> MGFKSWITEKLNPGQRIIRDMEPVSHRTNRKPFTTGQAYSKIEILNRTANMVIDSAAECSYTVGDKYNIVTYANGVKTKTLDTLLNVRPNPFMDISTFRRLVVTDLLFEGCAYIYWDGTSLYHVPAALMQVEADANKFIKKFIFNNQINYRVDEIIFIKDNSYVCGTNSQISGQSRVATVIDSLEKRSKMLNFKEKFLDNGTVIGLILETDEILNKKLRERKQEELQLDYNPSTGQSSVLILDGGMKAKPYSQISSFKDLDFKEDIEGFNKSICLAFGVPQVLLDGGNNANIRPNIELFYYMTIIPMLNKLTSSLTFFFGYKITPNTKEVAALTPDKEAEAKHLTSLVNNGIITGNEAR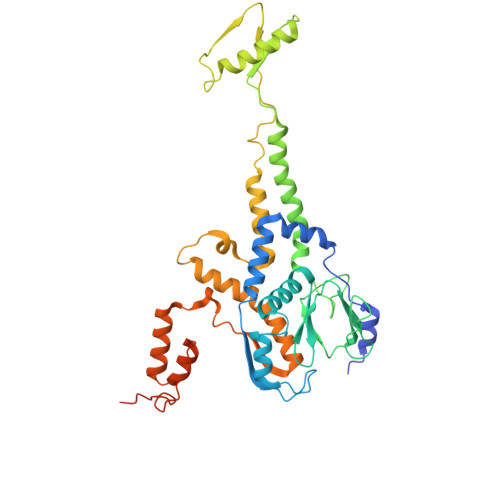SELNLEPLDDEQMNKIRIPANVAGSATGVSGQEGGRPKGSTEGD> ARSTNTFNYATYHTLDEIYDFMDLLVAEHPQLVSKLQIGRSYEGRPIYVLKFSTGGSNRPAIWIDLGIHSREWITQATGVWFAKKFTENYGQNPSFTAILDSMDIFLEIVTNPNGFAFTHSENRLWRKTRSVTSSSLCVGVDANRNWDAGFGKAGASSSPCSETYHGKYANSEVEVKSIVDFVKNHGNFKAFLSIHSYSQLLLYPYGYTTQSIPDKTELNQVAKSAVAALKSLYGTSYKYGSIITTIYQASGGSIDWSYNQ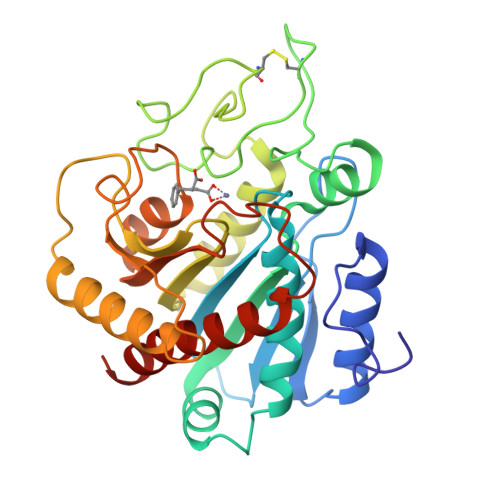GIKYSFTFELRDTGRYGFLLPASQIIPTAQETWLGVLTIMEHTVNN>[28x]MNLIPTVIETTNRGERAYDIYSRLLKDRIIMLGSQIDDNVAN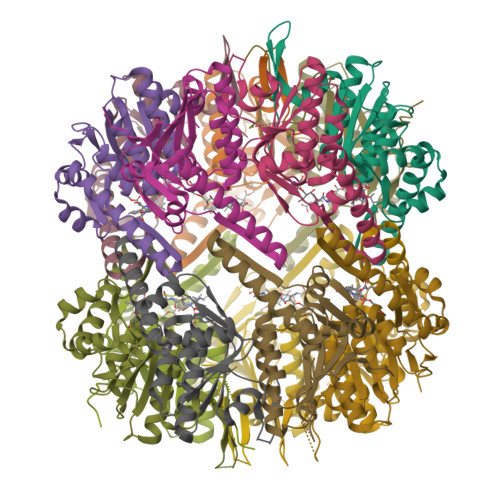SIVSQLLFLQAQDSEKDIYLYINSPGGSVTAGFAIYDTIQHIKPDVQTICIGMAASMGSFLLAAGAKGKRFALPNAEVMIHQPLGGAQGQATEIEIAANHILKTREKLNRILSERTGQSIEKIQKDTDRDNFLTAEEAKEYGLIDEVMVPETKWSHPQFEK> GSHMQALSYR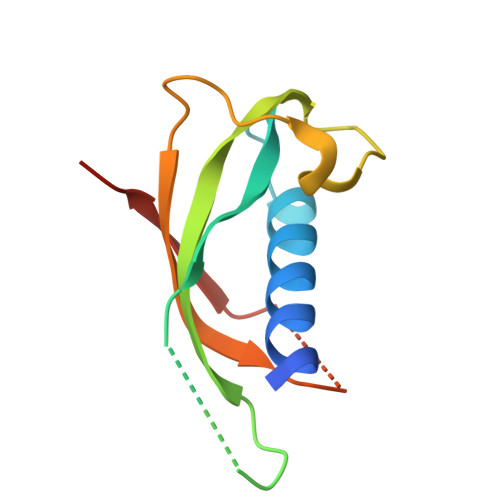EAVLRAVDRLNEQSSEANLYRLLELDQPPKADEDPGTPKPVSFTVKETVUPRPTRQPPELUDFKENGRVKQUVGTVTLDQIKDPLDITUNEVQGV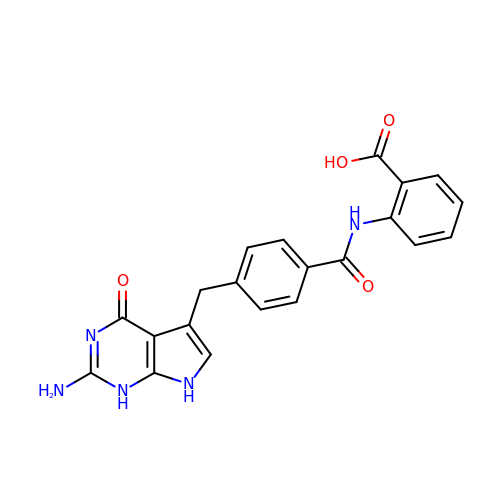2-({4-[(2-amino-4-oxo-4,7-dihydro-1H-pyrrolo[2,3-d]pyrimidin-5-yl)methyl]benzene-1-carbonyl}amino)benzoic acid | C21 H17 N5 O4 | NQGAZNWSUPTLIO-UHFFFAOYSA-N> MSKYSQDVLQLLYKNKPNYISGQSIAESLNISRTAVKKVIDQLKLEGCKIDSVNHKGHLLQQLPDIWYQGIIDQYTKSSALFDFSEVYDSIDSTQLAAKKSLVGNQSSFFILSDEQTKGRGRFNRHWSSSKGQGLWMSVVLRPNVAFSMISKFNLFIALGIRDAIQHFSQDEVKVKWPNDIYIDNGKVCGFLTEMVANNDGIEAIICGIGINLTQQLENFDESIRHRATSIQLHDKNKLDRYQFLERLLQEIEKRYNQFLTLPFSEIREEYNAASNIWNRTLLFTENDKQFKGQAIDL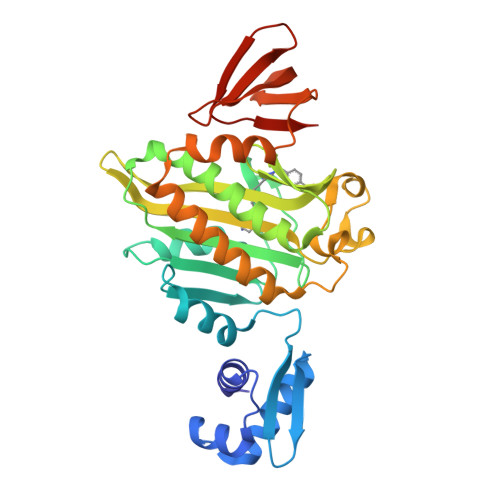DYDGYLIVRDEAGESHRLISADIDFHHHHHH> MKKGHHHHHHGSERTGTQPLGVQGLTEEQRMMIRELMDAQMKTFDTTFSHFKNFRLPGVLSSGCELPESLQAPSREEAAKWSQVRKDLCSLKVSLQLRGEDGSVWNYKPPADSGGKEIFSLLPHMADMSTYMFKGIISFAKVISYFRDLPIEDQISLLKGAAFELCQLRFNTVFNAETGTWECGRLSYCLEDTAGGFQQLLLEPMLKFHYMLKKLQLHEEEYVLMQAISLFSPDRPGVLQHRVVDQLQEQFAITLKSYIECNRPQPAHRFLFLKIMAMLTELRSINAQHTQRLLRIQDIHPFATPLMQELFGITGSLVPR

The human pregnane X receptor (PXR, NR1I2) is a transcription factor belonging to the nuclear receptor (NR) family. Indeed, the PXRLBD contains a large and versatile ligand-binding pocket (LBP), which enables it to bind a range of molecules with different structures and chemical properties, thereby fulfilling its biological functions. PXR is traditionally regarded as a xenobiotic receptor, and as such it regulates the transcription of metabolizing enzymes and drug transporters, thereby facilitating the removal of xenobiotics from the body. To overcome this problem, we designed a new PXRLBD-Thb-SRC-1 fusion construct that combines the advantage of having good stability and solubility during purification with the possibility of crystallizing the PXRLBD with or without SRC-1 thanks to the introduction of a thrombin cleavage site between the PXRLBD and SRC-1 parts.

In this context, we have also tested the hydrophobic tagging technology (HyT-technology), whereby proteins become unstable and are subsequently degraded by the proteasome following the addition of a hydrophobic group (for example adamantane) to their surface. Two new synthetic compounds, named JMV6995 and JMV7035, have been developed for this purpose. The difference between the two lies in the size and the chemical nature of the linker, with JMV7035 containing an additional PEG spacer. JMV6995 and JMV7035 were co-crystallized with the PXRLBD and were unambiguously positioned in the electron density of the resulting structures determined at 2.50 and 2.00 Å resolution, respectively. JMV6995 and JMV7035 mainly interact with the PXRLBD through van der Waals and hydrophobic contacts. Only one hydrogen bond is observed to the side chain of Ser247. In both cases, the mesityl sulfonamide group of the PXR agonist moiety is situated between helices H3 and H11, in close proximity to H12. On the other side of the pocket, the benzyl group is embedded within the aromatic π-trap, which is formed by Phe288, Trp299 and Tyr306.>MHHHHHHANLTGNVYIDGLWLPGHGAPFESVQPVTGETVWDGNAASLEDVDAAVREARKAFLAWRRKSLAERQAVIEAFGELLEANKEELAHQIGLETGKPLWESRTEVAAMMGKIPISVKAYNERTGHTESDVAGGHAVLRHRPHGVVAVFGPYNFPGHLPNGHIVPALLAGNTVVFKPSELTPGVAELTVRLWEKAGLPDGVINLVQGGSDTGKCLARHSLIDGLFFTGSSTVGHLLHEQFGGQPEKILALEMGGNNPLIVQNVSDLDGAVHHALQSAFLSAGQRCTCARRLLVPKGKKGDEFLARLVEVAARITVAEFDADPQPFMGSVISAEAANQLLKAQAAMLEKGA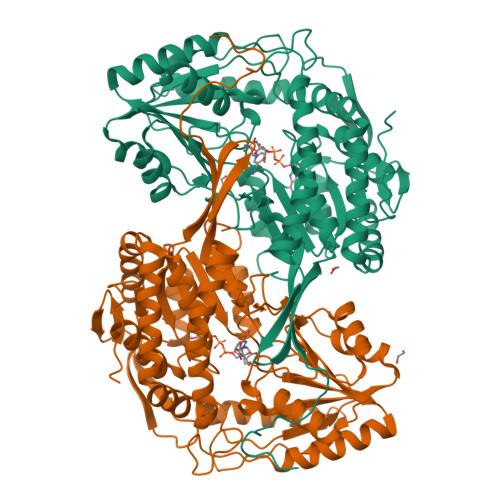TSLLEMKQLKPDTGLLSPGIVDATGIELEDQEFFGPLLTVYRYKGFDEALELANNTRYGLSAGILSDDRKLYNRLVEEVRAGIVNWNRPLTGASSAAPFGGVGASGNHRPSAYYAADYCAWPMASLEAGKSELPDSLAPGLNFD[2x]>[2x]TGQFSKTCEDITLDGSTLSAFCQKADGYTLNETSI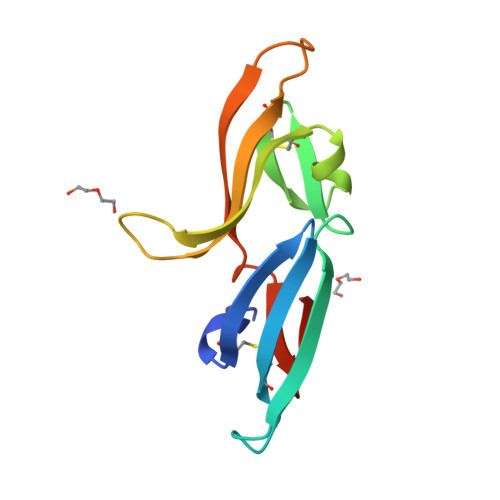NLDEEIGNLDGTLSWGDHNFSLTCDSIGLAQSLFTRTYVLAAECERRDGYTYIPTEIELDEHIANIDGTLTYE>MNIDLKGKVAVVSGGATLIGKAVVQALVSAGAHVAILDIDAKGKAIAESFNHDVMFIQTDLTSDAAIQQAVADIHQHLGEVSYLVNLACTYLDDGFKSSRQDWLQALDINLVSTVELSRALYNDLKKQQGSIVNFTSISAKVAQTGRWLYPVSKAAIRQLTQSMAMDFAADGIRVNSVSPGWTWSRVIAEVSGNNREKADSVAADYHLLGRLGHPEEVANVVLFLLSSAASFVTGADYAVDGGYSVMGPEGLQPAIPRLAE[2x]

Short-chain dehydrogenase/reductase enzymes are a large protein family with >60,000 members involved in numerous biosynthesis pathways. The short-chain dehydrogenase/reductase family, consisting of 60,000 documented enzymes, carry out the catalysis of oxidation/reduction reactions using either nicotinamide adenine dinucleotide (NADH) or nicotinamide adenine dinucleotide phosphate (NADPH) as a co-factor. SDR families share several standard features, despite sharing low sequence similarities (less than 30%), including the Rossman fold domain and the active site, consisting of a highly conserved tyrosine, lysine, serine, and often an asparagine. Here, an SDR family member from A. baumannii (Uniprot ID: A0A0M3FP68) was cloned, expressed, purified, and crystallised.

Crystals diffracted to 2.4 Å, permitting structure determination. During protein purification, the purity at each step was assessed by SDS-PAGE, and the sharp elution peak from the size exclusion column corresponded to a molecular weight of about 100 kDa, suggesting the enzyme was a tetramer (27 kDa protomer). Each monomer contains a central β -sheet (β1- β7), sandwiched between two groups of α- helices (α1-α2-α12-α13 and α3-α5-α6-α7-α8-α9-α10), with an overall topology of β1-α1-β2-α2-β3-α3-β4-α4-α5-α6-α7-β5-α8-α9-α10-β6-α11-α12-α13-β7-α14. After structural elucidation it was discovered that Gln69 was missing, and investigation revealed this error was introduced in the original design of the plasmid. Fortunately, overlay of the experimentally determined structure with the Gln69 deletion and the alpha fold prediction without the Gln69 deletion showed that the overall structure was not affected, and it overlayed perfectly with previously determined SDR structures. The structure presented in this study presented no evidence of the cofactor (or substrate) bound in the well described binding pocket. All four catalytic residues, previously characterised to have catalytic function in SDRs, are conserved in the SDR structure determined in this study (Asn108, Ser136, Tyr150, Lys153). In further support that NADH is more likely to be the cofactor rather than NADPH, superposition revealed a clash between the phosphate of NADPH and the loop between 38DIDAK42. This analysis also revealed that uniquely, the C-terminus of the SDR in this study, spanning residues 246VMGPEGLQPAIPRLAE261 extended diagonally and bound the adjacent protomer by interacting with loop regions 186–248, a region that plays a role in cofactor and substrate binding. Specifically, this interaction was mediated by Val246 hydrogen bonding with Ala143, Glu250 hydrogen bonding with Gln144, and Ala260 hydrogen bonding with Lys198, as well as a salt bridge interaction between Arg258 and Asp205.5,7-dihydroxy-2-(4-hydroxyphenyl)-4-oxo-4H-chromen-3-yl 3,4-di-O-acetyl-6-deoxy-alpha-L-mannopyranoside 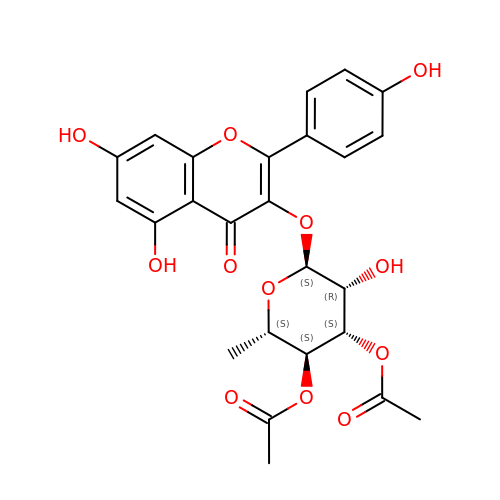| C25 H24 O12 | SXOZSDJHGMAEGZ-IGKKHSBFSA-N>MSQTHKHAIPANIADRCLINPEQYETKYKQSINDPDTFWGEQGKILDWITPYQKVKNTSFAPGNVSIKWYEDGTLNLAANCLDRHLQENGDRTAIIWEGDDTSQSKHISYRELHRDVCRFANTLLDLGIKKGDVVAIYMPMVPEAAVAMLACARIGAVHSVIFGGFSPEAVAGRIIDSSSRLVITADEGVRAGRSIPLKKNVDDALKNPNVTSVEHVIVLKRTGSDIDWQEGRDLWWRDLIEKASPEHQPEAMNAEDPLFILYTSGSTGKPKGVLHTTGGYLVYAATTFKYVFDYHPGDIYWCTADVGWVTGHSYLLYGPLACGATTLMFEGVPNWPTPARMCQVVDKHQVNILYTAPTAIRALMAEGDKAIEGTDRSSLRILGSVGEPINPEAWEWYWKKIGKEKCPVVDTWWQTETGGFMITPLPGAIELKAGSATRPFFGVQPALVDNEGHPQEGATEGNLVITDSWPGQARTLFGDHERFEQTYFSTFKNMYFSGDGARRDEDGYYWI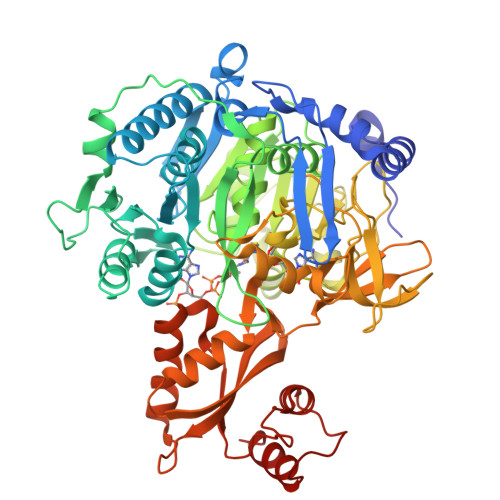TGRVDDVLNVSGHRLGTAEIESALVAHPKIAEAAVVGIPHAIKGQAIYAYVTLNHGEEPSPELYAEVRNWVRKEIGPLATPDVLHWTDSLPKTRSGKIMRRILRKIAAGDTSNLGDTSTLADPGVVEKLLEEKQAIAMPS[2x]> GSTVQVP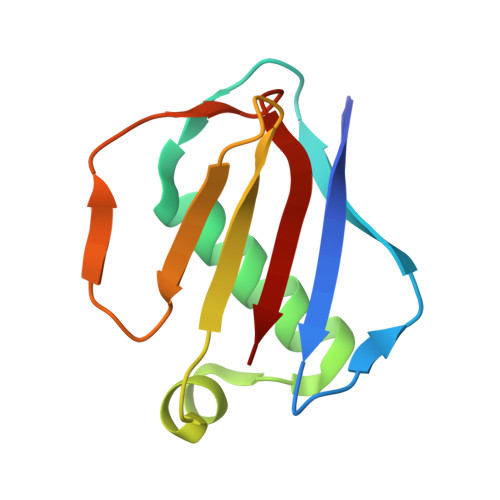YTITVNGTSQNILSNLTFNKNQNISYKDLEGKVKSVLESNRGITDVDLRLSKQAKYTVNFKNGTKKVIDLKSGIYTANLINSSDIKSININVD> MSAAIAEPTSHDPDSGGHFGGPSGWGGRYVPEALMAVIEEVTAAYQKERVSQDFLDDLDRLQANYAGRPSPLYEATRLSQHAGSARIFLKREDLNHTGSHKINNVLGQALLARRMGKTRVIAETGAGQHGVATATACALLGLDCVIYMGGIDTARQALNVARMRLLGAEVVAVQTGSKTLKDAINEAFRDWVANADNTYYCFGTAAGPHPFPTMVRDFQRIIGMEARVQIQGQAGRLPDAVVACVGGGSNAIGIFHAFLDDPGVRLVGF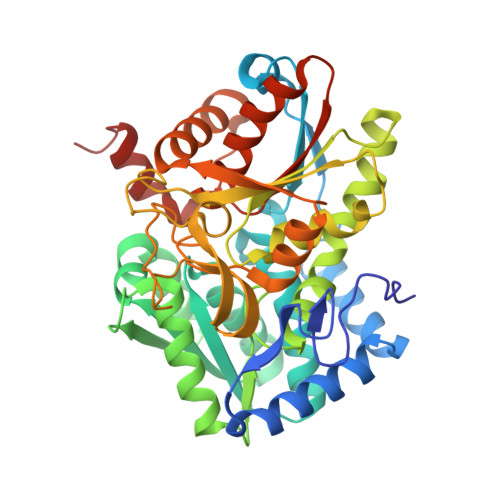EAAGDGVETGRHAATFTAGSPGAFHGSFSYLLQDEDGQTIESHSISAGLDYPGVGPEHAWLKEAGRVDYRPITDSEAMDAFGLLCRMEGIIPAIESAHAVAGALKLGVELGRGAVIVVNLSGRGDKDVETAAKWFGLLGND> MKFFDGVKDVLSGLINRRNSMARNRVSHRYLSDEEMRVMYKAGLMSKIIRLKAGYALNDTLKFESTQDQEIYKKRLSKHVKNATKFMLGFGRGVIVVFKNGDDLSKPLERGVDPKLLKIRVFSGDIAKGNNPDNDLRSERYYKPKNYTIKGHTIHWTRVVDFTYYMPSENELPDYYYGGMSESELIYEQFINDSVVQRASGSIIEKASTFVYKIKGYKQLIQAKKEEDIIKYVSTCEDGRSIYGGLITDADDEVSTLTQSLTDLDKVDNVTLRRIAMVTGLGMTVLIGEQASGLNASGEKERQGFQDTIENLQSDYLEDPLNRLAEIFQLGFI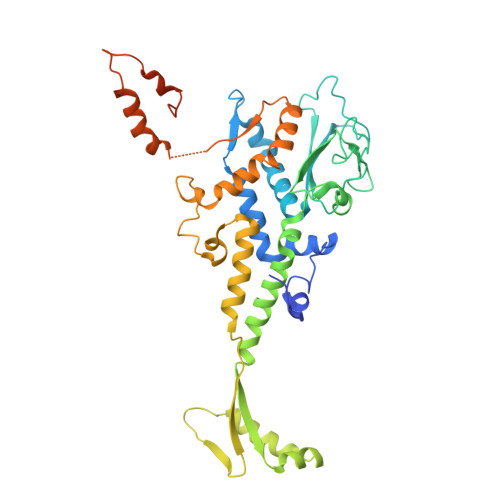EFKDNQGQSANERVEYDKKAVDVAKVLWELGEDYGAYLKDKDVVQADDWDNFWKEKDENSEVDESLPLGDLFSSGDVNG> MAKEWGYASHNGPDHWHELFPNAKGENQSPIELHTKDIRHDPSLQPWSVSYDGGSAKTILNNGKTCHVVFDDTYDRSMLRGGPLPGPYRLRQFHLHWGSSDDHGSEHTVDGVKYAAELHLVHWNPKYNTFKEALKQRDGIAVIGIFLKIGHENGEFQIFLDALDKIKTKGKEAPFTKFDPSSLFPASRDYWTYQGSFTTPPCEECIVWLLLKEPMTVSSDQMAKLRSLLSSAENEPPVPLVSNWRPPQPINNR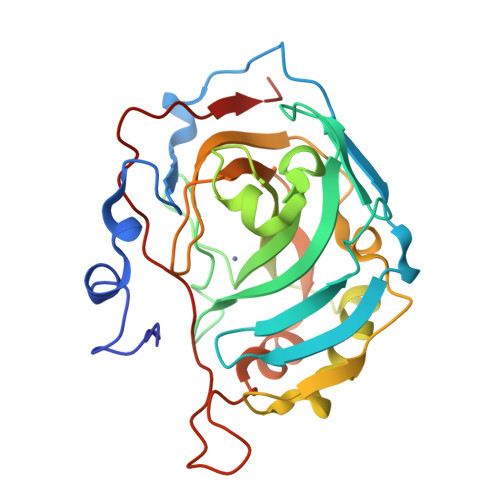VVRASFK Syntenin-1, a member of the PDZ domain-containing scaffold protein family, is involved in diverse physiological processes, such as cell adhesion, protein trafficking10, and transcription factor activation. Syntenin-1 is an adaptor-like molecule that contains at least four separate structural domains: An N-terminal domain, two tandem PDZ domains (PDZ1 and PDZ2), and a C-terminal region. The diverse biological functions of syntenin-1 arise from its ability to bind the cytoplasmic domains of numerous physiologically relevant signaling and adhesion molecules, including syndecans, neurexins, and ephrin B12131415. The present study provides clear evidence that syntenin-1 negatively regulates syndecan-4 signaling via binding between syndecan-4 and the syntenin-1 PDZ2 domain.

The crystal structures of syntenin-1 with and without a syndecan-4 cytoplasmic domain peptide (corresponding to the C2 region; 4C2) were determined to be 2.8 and 1.9 Å, respectively. In our structural superpositioning of syntenin-1/4C2 with syntenin-1, the overall RMSD was 1.493 Å. In the absence of syndecan-4 however, the molecular surface of PDZ2 in the syntenin-1/4C2 complex was wider than that of syntenin-1. Upon syndecan-4 binding, a structural rearrangement of the PDZ2 domain provided a specific binding pocket for the syndecan-4 cytoplasmic domain. Indeed, both pull-down assays and gel filtration chromatography showed that syntenin-1 exists as a dimer under physiological conditions. Our structural analysis showed that four residues (Q162 and A169 in PDZ1; R193 and F197 in the linker region) were involved in dimeric interactions with four PDZ2 residues (R199, N232, A230, and R231). Notably, both electrostatic and hydrophobic interactions contribute to the dimerization of syntenin-1.

>[2x]GSAMADIGAEIKQGIREVILCKDQDGKIGLRLKSVDNGIFVQLVQANSPASLVGLRFGDQVLQINGENCAGWSSDKAHKVLKQAFGEKITMTIRDRPFERTVTMHKDSSGHVGFIFKSGKITSIVKDSSAARNGLLTDHHICEINGQNVIGLKDAQIADILSTAGTVVTITIMPAFIFEHIIKRMAPSIMKSLMDHTIPEV Mammals depend on dietary uptake of Cobalamin (Cbl), which is a cofactor of at least two enzymes that are part of essential biochemical pathways. CD320 is a member of the Low-density Lipoprotein Receptor (LDLR) family, a large group of mostly multi-ligand receptors involved in cholesterol uptake and other physiologically essential functions. CD320 features an N-terminal, extracellular fragment comprising two LDLR type A (LDLR-A) domains separated by an epidermal growth factor (EGF) homology domain, the exact function of which has so far not been determined. While the majority of related LDLR domain-containing receptors bind multiple and distinct ligands, CD320 has been reported to bind TC with high specificity and affinity as evidenced by the lack of interference in TC binding from related LDLR ligands like LDL and RAP as well as high affinity for TC of both the full-length receptor and its soluble ectodomain81318.

Deletion of a single glutamate (ΔE88) in LDLR-A1 of CD320 has been associated with Cbl deficiency observed in patients carrying the mutation. To investigate whether a structural effect was underpinning this defect, we generated a complex of TC with CD320ΔE88, characterized it biochemically and determined its structure at 2.6 Å resolution. However, the purified complex displayed increased propensity to form non-specific multimers as analysed by SEC, requiring an additional SEC purification step for crystallization. As the mutant complex structure was of lower resolution than that of the wild type, we confirmed the positions of disulfide bonds and bound Ca2+ ions by using anomalous difference peaks from data collected at a wavelength of 1.77 Å. The TC-CD320ΔE88 structure revealed a similar domain arrangement and binding interface as the wild-type protein and we observed no significant changes in TC or the LDLR-A2 domain, ruling out a gross structural effect of the ΔE88 mutation. As seen for the wild-type protein, the region of LDLR-A1 carrying the deletion (EEE loop) revealed poor electron density and higher B-factors when compared with that of LDLR-A2 (average B-factors for LDLR-A1 and A2 Ca2+ ions ∼112 and 56 Å2, respectively). Moreover, electron density for the Ca2+ binding residue Glu86 as well as Glu87 and disulfide forming Cys88 (equivalent to Cys89 in wild type) was missing. However, the centrally bound Ca2+ as well as the LDLR-A1 acidic necklace was clearly visible in our structure indicating intact Ca2+ binding. Even though the apparent Tm of the complex was slightly lower than that of the wild-type protein, approaching that of the LDRL-A2 domain alone, the mutant protein bound TC with equivalent affinity to wild type with a calculated KD of 1.5 nM. At least in vitro, these findings rule out a compromised ability of CD320ΔE88 to bind TC.

>EMCEIPEMDSHLVEKLGQHLLPWMDRLSLEHLNPSIYVGLRLSSLQAGTKEDLYLHSLKLGYQQCLLGSAFSEDDGDCQGKPSMGQLALYLLALRANCEFVRGHKGDRLVSQLKWFLEDEKRAIGHDHKGHPHTSYYQYGLGILALCLHQKRVHDSVVDKLLYAVEPFHQGHHSVDTAAMAGLAFTCLKRSNFNPGRRQRITMAIRTVQEEILKAQTPEGHFGNVYSTPLALQFLMTSPMRGAELGTACLKARVALLASLQDGAFQNALMISQLLPVLNHKTYIDLIFPDCLAPRVMLEPAAETIPQTQEIISVTLQVLSLLPPYRQSISVLAGSTVEDVLKKAHELGGFTYETQASLSGPYLTSVMGKAAGEREFWQLLRDPNTPLLQGIADYRPKDGETIELRLVSW[2x];>[2x]SCPPTKFQCRTSGLCVPLTWRCDRDLDCSDGSDEECRIEPCTQKGQCPPPPGLPCPCTGVSDCSGGTDKKLRNCSRLACLAGELRCTLSDDCIPLTWRCDGHPDCPDSSDELGCGTNE> AEETCFDKYTGNTYRVGDTYERPKDSMIWDCTCIGAGRGRISCTIANRCHEGGQSYKIGDTWRRPHETGGYMLECV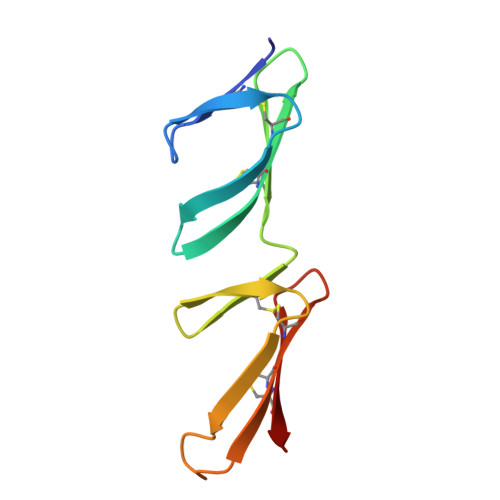CLGNGKGEWTCKPI> MLRCTVVGHHRSGKARAFVFRDPSLRMMRAGSGYQQLRRMGMPMQVGMGWRKVDSFHANTQYQHAWPLLSHDDLGNSDQSNNTKNIMYSMYMPKRNKGTAPWFRGADTYSVKYCEQGRYEYQRYLMINRFPSEYKKHFLSFLSNIRMSSGSATIPQEALHWLLRMIVDNFNPQHVHYIAAMKTLQSAGELDMARDVWKIMERQQTWPCTATICAYLDVCVEAGEKTWAMEAWNRYCTELKFLEPGEVDPKPISRVPFSLTREELLYLPKWKKHFDHDPNLDVMDLNRFNRTREVYLRMAQVMLAGGE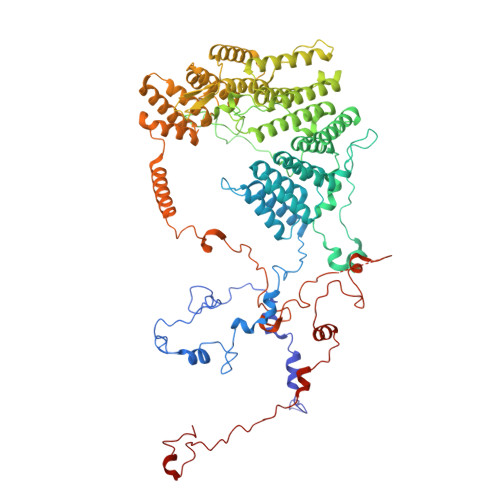RNAFQHFFTKLEEAMLNKPTPVPEPPNPHLVRRPRWAPYEHCKSVHHSPWRLQNNGRALALGPPVTIEDEMQSRFFSNDQFLVHSVKEVLRIVLQEHKRAHPTECTRCKTEAFFYKTKDADETLKFCDDLIERLFASLGVRLSNLNTSSLLSTILEVFRVVGKESGAALLQRANEFLERKASLGDAEGSRENLTASNYLQVLSGFADESAFVYNTKKDGTCQYKTGFDPRTTMRHLADVVQEIAGNPHVTWAADMHLQVVETMVGCGTMKANDYFVRNVLRQFSWDSRFLEALYVEYRRQDDVDMWAELTKRALVWTARYNAPASERLRRLIEDDYDTIRVQTRTFRELAVFQFRDVEERRHSRDVVNELPNPWYDYVAHALPFPDRDAGYPDEYGDLGQWRAPGGPGSPVRGPGYYAPPMEGEHQRGYTAEWRDLRNPMRPPEFPTPWERKYRQYARGQHPSYDMVYAGPMPEIFPMRRDFRKPTRWDFHDIEKQGKYRTSGPY> GSADAPRDRHRTIVVGGDRDYPPYEFIDQNGKPAGYNVELTRAIAEVMGMTVEFRLGAWSEMFSALKSGRVDVLQGISWSEKRARQIDFTPPHTIVYHAIFARRDSPPAAGLEDL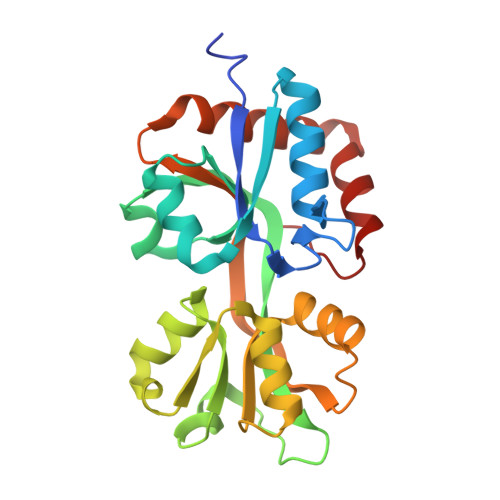RGRKVALHRDGIMHEYLAERGYGKDLVLTPTPADALRLLAAGGCDYAVVAMVPGMYIIRENRLTNLVPVARSIAAQRYGYAVRQGDAELLARFSEGLAILRKTGQYEAIRAKWLGVLEP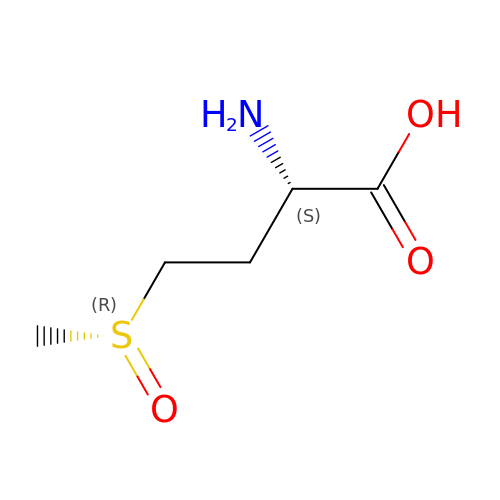METHIONINE SULFOXIDE | C5 H11 N O3 S | QEFRNWWLZKMPFJ-ZXPFJRLXSA-N> MELSPTYQTERFTKFSDTLKEFKIEQNNEQNPIDPFNIIREFRSAAGQLALDLANSGDESNVISSKDWELEARFWHLVELLLVFRNADLDLDEMELHPYNSRGLFEKKLMQDNKQLYQIWIVMVWLKENTYVMERPKNVPTSKWLNSITSGGLKSCDLDFPLRENTNVLDVKDKEEDHIFFKYIYELILAGAIDEALEEAKLSDNISICMILCGIQEYLNPVIDTQIANEFNTQQGIKKHSLWRRTVYSLSQQAGLDPYERAIYSYLSGAIPNQEVLQYSDWESDLHIHLNQILQTEIENYLLENNQVGTDELILPLPSHALTVQEVLNRVASRHPSESEHPIRVLMASVILDSLPSVIHSSVEMLLDVVKGTEASNDIIDKPYLLRIVTHLAICLDIINPGSVEEVDKSKLITTYISLLKLQGLYENIPIYATFLNESDCLEACSFILSSLEDPQVRKKQIETINFLRLPASNILRRTTQRVFDETEQEYSPSNEISISFDVNNIDMHLIYGVEWLIEGKLYVDAVHSIIALSRRFLLNGRVKALEQFMERNNIGEICKNYELEKIADNISKD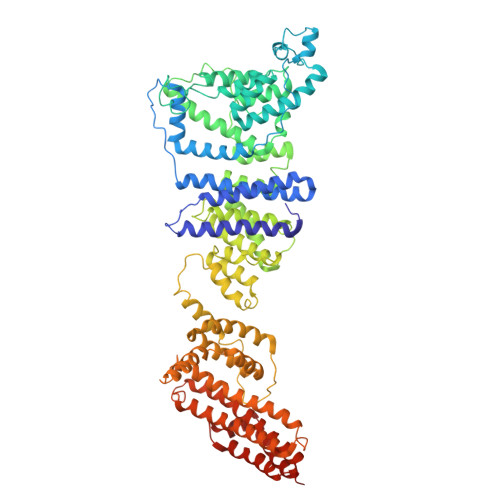ENEDQFLEEITQYEHLIKGIREYEEWQKSVSLLSSESNIPTLIEKLQGFSKDTFELIKTFLVDLTSSNFADSADYEILYEIRALYTPFLLMELHKKLVEAAKLLKIPKFISEALAFTSLVANENDKIYLLFQSSGKLKEYLDLVARTATLSN>GAMGSLIRKKAAGLESAATIRTKVFVWGLNDKDQLGGLKGSKIKVPSFSETLSALNVVQVAGGSKSLFAVTVEGKVYACGEATNGRLGLGISSGTVPIPRQITALSSYVVKKVAVHSGGRHATALTVDGKVFSWGEGDDGKLGHFSRMNCDKPRLIEALKTKRIRDIACGSSHSAALTSSGELYTWGLGEYGRLGHGDNTTQLKPKMVKVLLGHRVIQVACGSRDAQTLALTDEGLVFSWGDGDFGKLGRGGSEGCNIPQNIERLNGQGVCQIECGAQFSLALTKSGVVWTWGKGDYFRLGHGSDVHVRKPQVVEGLRGKKIVHVAVGALHCLAVTDSGQVYAWGDNDHGQQGNGTTTVNRKPTLVQGLEGQKITRVACGSSHSVAWTTVDVATPSVHEPVLFQT[3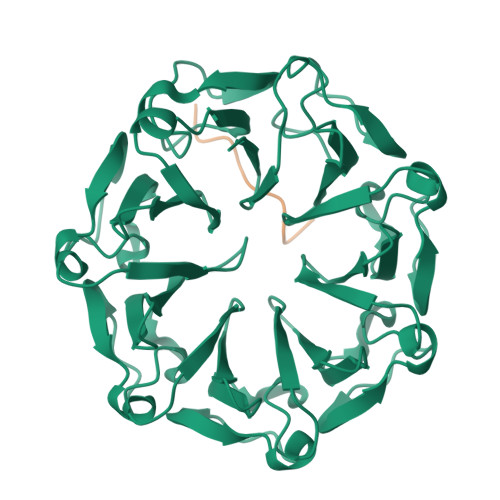x];>[3x]RSDDDKDEDTHSRK>AIFHTGSELFIITRGPGKLTLLTWGGLNNLRSVIGAIPTENTGVTKWAVSFSHNYTRFSFIWEGQGEACYQIGNGLTRSPVGRSWSSSSTIHWGS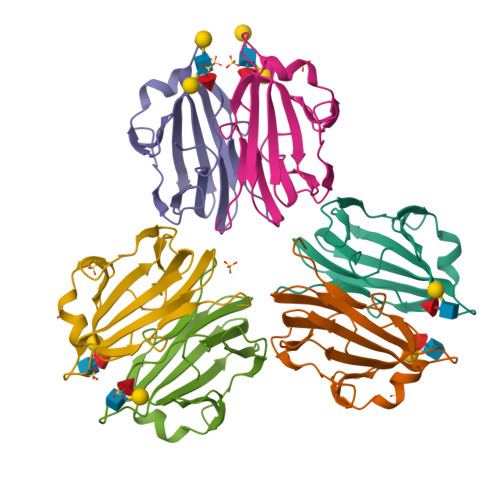STVITEDVTSVVPGAVNRDKVTTAYALPDNL[6x]>[2x]MKLKTTLFGNVYQFKDVKEVLAKANELRSGDVLAGVAAASSQERVAAKQVLSEMTVADIRNNPVIAYEDDCVTRLIQDDVNETAYNQIKNWSISELREYVLSDETSVDDIAFTRKGLTSEVVAAVAKICSNADLIYGAKKMPVIKKANTTIGIPGTFSARLQPNDTRDDVQSIAAQIYEGLSFGVGDAVIGVNPVTDDVENLSRVLDTIYGVIDKFNIPTQGCVLAHVTTQIEAIRRGAPGGLIFQSICGSEKGLKEFGVELAMLDEARA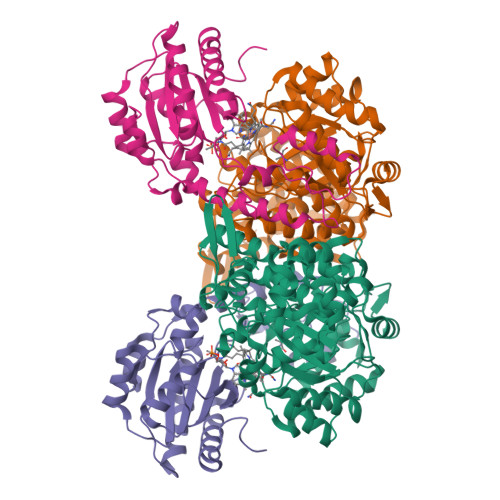VGAEFNRIAGENCLYFETGQGSALSAGANFGADQVTMEARNYGLARHYDPFIVNTVVGFIGPEYLYNDRQIIRAGLEDHFMGKLSGISMGCDCCYTNHADADQNLNENLMILLATAGCNYIMGMPLGDDIMLNYQTTAFHDTATVRQLLNLRPSPEFERWLESMGIMANGRLTKRAGDPSLFF;>MDQSSHHHHHHALDLGSAEAKAWIGVENPHRADVLTELRRSTVARVCTGRAGPRPRTQALLRFLADHSRSKDTVLKEVPEEWVKAQGLLEVRSEISDKNLYLTRPDMGRRLCAEAVEALKAQCVANPDVQVVISDGLSTDAITVNYEEILPPLMAGLKQAGLKVGTPFFVRYGRVKIEDQIGEILGAKVVILLVGERPGLGQSESLSCYAVYSPRMATTVEADRTCISNIHQGGTPPVEAAAVIVDLAKRMLEQKASGINMTR[2x]>GSHMTQQIKLLVLNGPNLNLLGQREPEVYGSKTLDDIIKALTDEAALQNVALSHLQSNREYELIEKIHDAFEKIDFIIINPAAFTHTSVALRDALLGVNIPFIEVHLSNVHARESFRH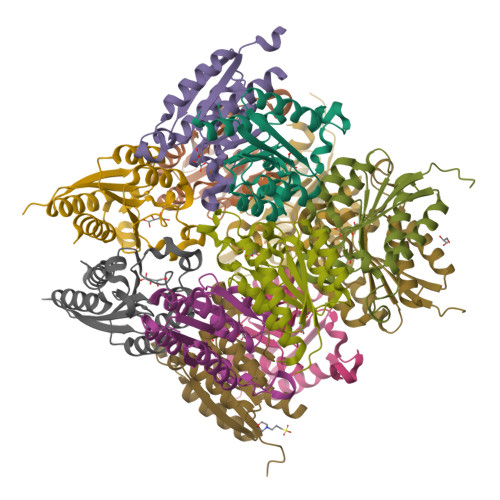HSYLSDIAQGVICGLGAKGYSFALQSAIGKLRNI[12x]>[3x]MRIVAADTGGAVLDESFQPVGLIATVAVLVEKPYKTSKRFLVKYADPYNYDL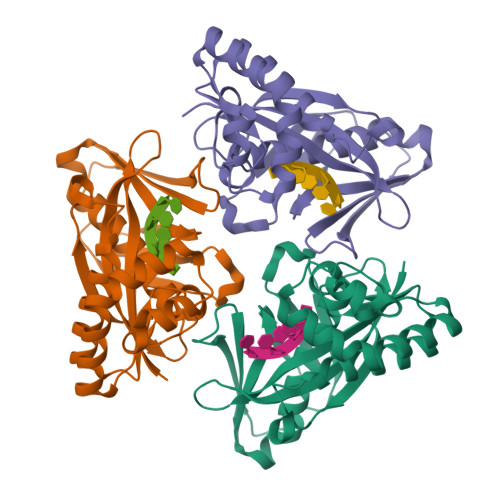SGRQAIRDEIELAIELAREVSPDVIHLNSTLGGIEVRKLDESTIDALQISDRGKEIWKELSKDLQPLAKKFWEETGIEIIAIGKSSVPVRIAEIYAGIFSVKWALDNVKEKGGLLVGLPRYMEVEIKKDKIIGKSLDPREGGLYGEVKTEVPQGIKWELYPNPLVRRFMVFEITSKSHHHH2-oxidanyl-4-phenyl-benzoic acid | C13 H10 O3 | 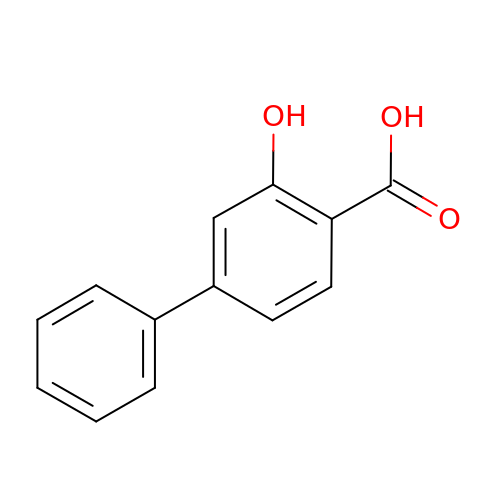IDXMMAOAJXZWSS-UHFFFAOYSA-N> KEQRLKEQLGAQQEPVKKSIQESEAFLPQSIPEERYKMKSKPLGICLIIDCIGNETELLRDTFTSLGYEVQKFLHLSMHGISQILGQFACMPEHRDYDSFVCVLVSRGGSQSVYGVDQTHSGLPLHHIRRMFMGDSCPYLAGKPKMFFIQNYVVSEGQLENSSLLEVDGPAMKNVEFKAQKRGLCTVHREADFFWSLCTADM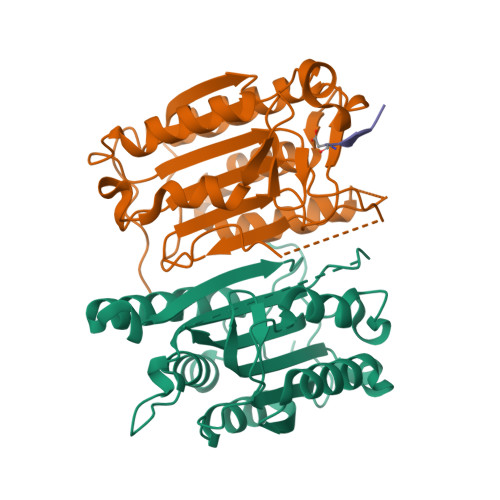SLLEQSHSSPSLYLQCLSQKLRQERKRPLLDLHIELNGYMYDWNSRVSAKEKYYVWLQHTLRKKLILSYT;> SESQTLDKVYQMKSKPRGYCLIINNHNFAKAREKVPKLHSIRDRNGTHLDAGALTTTFEELHFEIKPHDDCTVEQIYEILKIYQLMDHSNMDCFICCILSHGDKGIIYGTDGQEAPIYELTSQFTGLKCPSLAGKPKVFFIQACQGDNYQKGIPVETASEEQPYLEMALSSPQTRYIPDEADFLLGMATVNNCVSYRNPAEGTWYIQSLCQSLRERCPRGDDILTILTEVNYEVSNKDDKKNMGKQMPQPTFTLRKKLVFPSDVEHHHHHH;> AIETD> MEYKSSPKRPYYLRGFYDWLVDNSFTPYLVVDATYLGVNVPVEYVKDGQIVLNLSASATGNLQLTNDFIQFNQRF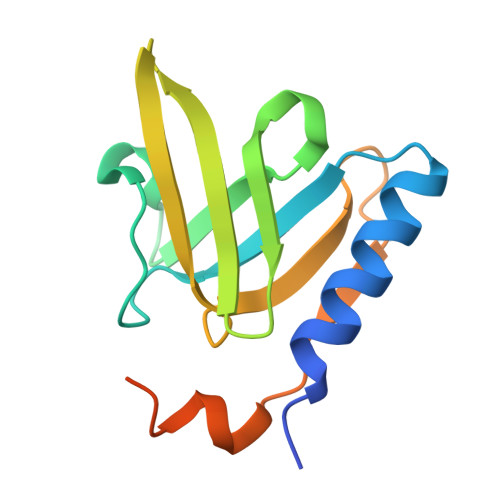KGVSRELYIPMGAALAIYARENGDGMMFEPEEIYDELNIEPDTEQPTGFYEAVD> MESKLNLDFNLVEKARAKAKAIAIDTQEFIEKHTTVTVERAVCRLLGIDGVDTDEVPLPNIVVDHIKENNGLNLGAAMYIANAVLNTGKTPQEIAQAISAGELDLTKLPMKDLFEVKTKALSMAKE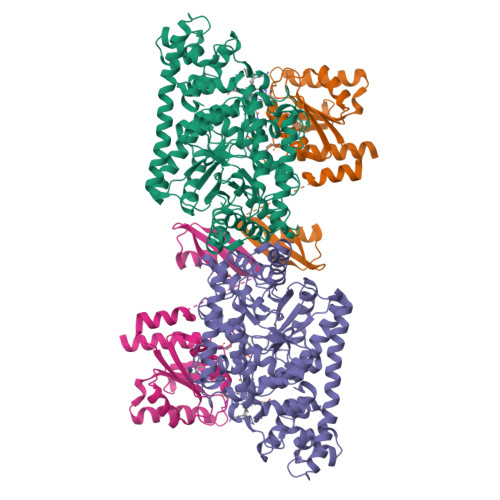TVEKIKNNRSIRESRFEEYGDKSGPLLYVIVATGNIYEDITQAVAAAKQGADVIAVIRTTGQSLLDYVPYGATTEGFGGTYATQENFRLMREALDKVGAEVGKYIRLCNYCSGLCMPEIAAMGAIERLDVMLNDALYGILFRDINMQRTMIDQNFSRIINGFAGVIINTGEDNYLTTADAFEEAHTVLASQFINEQFALLAGLPEEQMGLGHAFEMDPELKNGFLYELSQAQMAREIFPKAPLKYMPPTKFMTGNIFKGHIQDALFNMVTIMTNQRIHLLGMLTEALHTPFMSDRALSIENAQYIFNNMESISEEIQFKEDGLIQKRAGFVLEKANELLEEIEQLGLFDTLEKGIFGGVKRPKDGGKGLNGVVSKDENYYNPFVELMLNK;> MSSGLYSMEKKEFDKVLDLERVKPYGDTMNDGKVQLSFTLPLKNNERSAEAAKQIALKMGLEEPSVVMQQSLDEEFTFFVVYGNFVQSVNYNEIHVEAVNSEILSMEETDEYIKENIGRKIVVVGASTGTDAHTVGIDAIMNMKGYAGHYGLERYEMIDAYNLGSQVANEDFIKKAVELEADVLLVSQTVTQKNVHIQNMTHLIELLEAEGLRDRFVLLCGGPRINNEIAKELGYDAGFGPGRFADDVATFAVKTLNDRMNS>GGSHDCAKVDLENAELRRKLIRTKRAFEDTYEKLRMANKAKAQVEKDIKNQILKTHNVLRNVRSNMENEL[4x];>GPMDQQNSAVIGQLRLELQQARTEVETADKWRLECIDVCSVLTNRLEEEAGFLNSLLK[4x]

In flies, Centrosomin (Cnn) forms a phosphorylation-dependent scaffold that recruits proteins to the mitotic centrosome, but how Cnn assembles into a scaffold is unclear. We show that scaffold assembly requires conserved leucine zipper (LZ) and Cnn-motif 2 (CM2) domains that co-assemble into a 2:2 complex in vitro. Purified CM2 forms a stable 2:2 tetramer with the purified LZ of the PReM domain, and we solve the crystal structure of the LZ:CM2 complex, revealing that helical dimers of LZ and CM2 interact in an anti-parallel fashion. Thus, Cnn molecules have an intrinsic ability to form large, LZ:CM2-interaction-dependent assemblies that are critical for mitotic centrosome assembly.

Most of these substitutions strongly perturbed the ability of the LZ to form a stable 2:2 tetramer with CM2, the only exception being L535E, which still formed a 2:2 tetramer but with reduced efficiency. The purified LZ-L535E protein exhibits reduced α helicity, suggesting that it is partially unfolded (red line), yet it can still interact with CM2. To better understand why the L535E substitution did not more strongly disrupt the LZ:CM2 interaction, we generated LZ-L535E:CM2 crystals and solved their structure. Perhaps surprisingly, LZ-L535E appeared to be folded normally and was largely helical within the crystal structure. Although L535 is packed within the core of the LZ:CM2 assembly, there is sufficient space in the core to accommodate the longer E535 side chain, and E535 also forms a hydrogen bond with the invariant CM2 T1133 residue in the core. This presumably explains why the L535E mutation only relatively mildly perturbs LZ:CM2 assembly in vitro and Cnn scaffold assembly in vivo.1,5-dimethyl-6-(2-oxidanyl-6-oxidanylidene-cyclohexen-1-yl)carbonyl-3-(4-phenylbutyl)quinazoline-2,4-dione | C27 H28 N2 O5 | 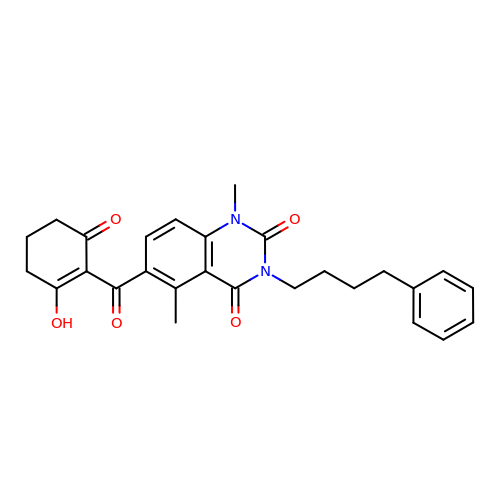JXJBJFQGJRQBHO-UHFFFAOYSA-N The bifunctional enzyme Δ1-pyrroline-5-carboxylate synthase (P5CS) is vital to the synthesis of proline and ornithine, playing an essential role in human health and agriculture. The P5CS molecule contains two domains, GK and GPR, catalyzing the first and second steps in the biosynthesis of proline from glutamate. The GK domain catalyzes glutamate phosphorylation, and the GPR domain catalyzes the NADPH-dependent reduction of γ-glutamyl phosphate (G5P) to glutamate-γ-semialdehyde (GSA). Our results describe the assembly mechanism of P5CS filaments, in which the GK domain forms tetramer and the GPR domain forms dimer structure, and both domains form specific interaction interfaces.

By focus refinement of the GPR dimer in the P5CSMix filament, we determined two additional states of the GPR domain. One is the NADP(H)-binding state, when NADP(H) is present at NBD. Upon NADP(H) binding, the residue R525 interacts with the adenine moiety. This interaction transforms the 525REE527 loop into an ordered structure that extends the α16 helix in the Rossmann-like fold. Meanwhile, the entire NBD rotates approximately 15° along the cylinder axis and slides towards CD. A similar phenomenon was also observed in ALDH1L1. This transformation contributes to bringing the nicotinamide ring of the NADP(H) close to the catalytic residue C598 of CD. Conformational changes triggered by the binding of NADPH subsequently initiate the transfer of the hydride ion from NADPH to the intermediate G5P. In our models, unliganded, G5P-binding and NADP(H)-released states represent as open conformation, and the NADP(H)-binding state represents as closed conformation. However, in the closed conformation, when the nicotinamide ring of NADP(H) approaches the G5P-binding site, the substrate tunnel entrance may be blocked by NADP(H). Next, NADPH binds to the GPR domain, triggering the conformational change into closed conformation, which brings the NADPH towards the catalytic residue C598 and facilitates the reaction.

> MLQNSFKLAQSLRNGFYRNAWRAFSSHGPRQPLVSPERRLEKAHPTFTERSQLKYARRLVVKLGSAVITREDNHGLALGRLASIVEQVAECHLEGREVMMVTSGAVAFGKQKLAQELLMSLSMRETLNPKDSKEFDGATLEPRAAAAVGQSGLMSLYDAMFAQYGVKIAQVLVTKPDFYNEETRNNLFCTLSELISLNIVPIINTNDAVSPPMFIRDDEPAGGARRGIPIKDNDSLSAMLAAEVQADLLILMSDVDGIYNKPPWEDGAKLMHTYTSDDSNSIEFGKKSKVGTGGMDSKVKAATWALDRGVSVVICNGMQEKAIKTIIGGRKVGTFFTEATESANAVPVEVMAENARTGSRQMQALTPAQRASAVNTLADLLVSREKFILDANAKDLAEAQKSGLAKPLLSRLSLNPAKLKNLSVGLKQIAEDSHKNVGRVLRRTRLADQLELKQVTVPIGVLLVIFESRPDSLPQVAALAMASANGLLLKGGKEAAHSNKALMELVKEALATVGAEHAVSLVSTREEISDLLSMENHIDLIIPRGSSDLVRSIQQQSLHIPVLGHAEGVCHVYIDRDADLEKALRIARDAKCDYPAACNAMETLLIHEDLMSGAIFGDVCNMLKREGVKIYAGPRLNQQLTFGPPAAKSLKHEYGALECCIEVVPSLDEAINHIHTYGSSHTDVIVTENDAAARQFLGSVDSACVFHNASSRFADGFRFGLGAEVGISTARIHARGPVGVEGLLTTKWILEGQDHAAADFAEGGGRTWLHETLPLD> GGGGGMNLSLSDLHRQVSRLVQQESGDCTGKLRGNVAANKETTFQGLTIASGARESEKVFAQTVLSHVANVVLT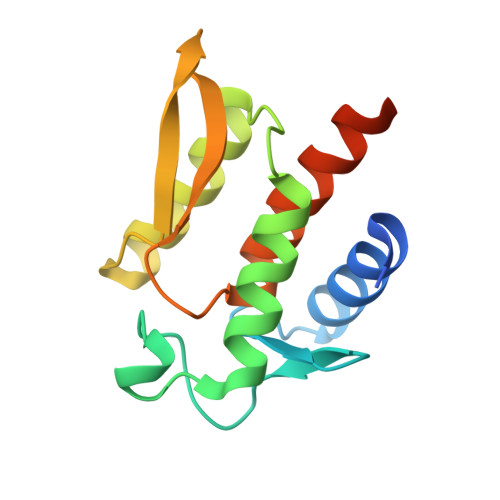QEDTAKLLQSTVKHNLNNYDLRSVGNGNSVLVSLRSDQMTLQDAKVLLEAALRQESGARGHHHHHH2-OXO-1,2,3,6-TETRAHYDROPYRIMIDINE-4,6-DICARBOXYLIC ACID | C6 H6 N2 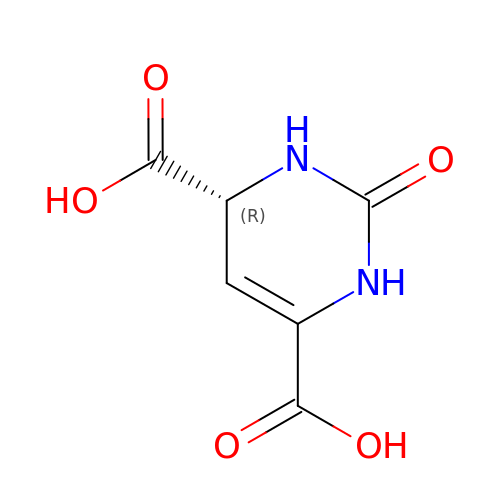O5 | WVCOMWPLPGATRR-UWTATZPHSA-N>MTKLDKG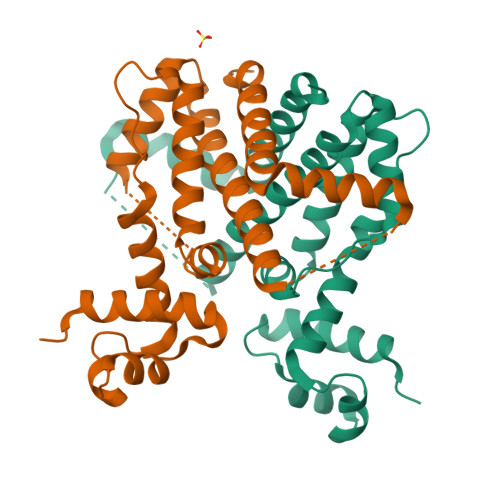TVIAAALELLNEVGMDSLTTRKLAERLKVQQPALYWHFQNKRALLDALAEAMLAERHTRSLPEENEDWRVFLKENALSFRTALLSYRDGARIHAGTRPTEPNFGTAETQIRFLCAEGFCPKRAVWALRAVSHYVVGSVLEQQASDADERVPDRPDVSEQAPSSFLHDLFHELETDGMDAAFNFGLDSLIAGFERLRSSTTDHHHHHH[2x]>STPSIVIASAARTAVGSFNGAFANTPAHELGATVISAVLERAGVAAGEVNEVILGQVLPAGEGQNPARQAAMKAGVPQEATAWGMNQLCGSGLRAVALGMQQIATGDASIIVAGGMESMSMAPHCAHLRGGVKMGDFKMIDTMIKDGLTDAFYGYHMGTTAENVAKQWQLSRDEQDAFAVASQNKAEAAQKDGRFKDEIVPFIVKGRKGDITVDADEYIRHGATLDSMAKLRPAFDKEGTVTAGNASGLNDGAAAALLMSEAEAS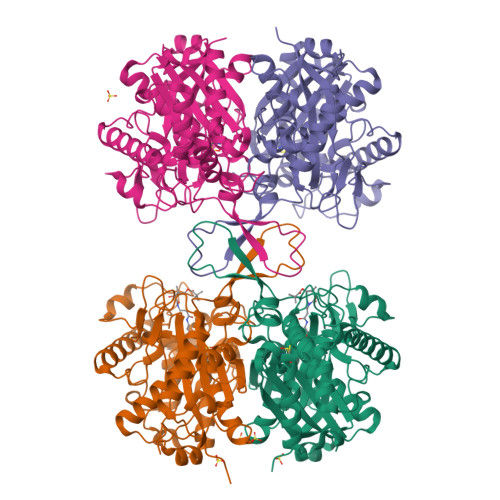RRGIQPLGRIVSWATVGVDPKVMGTGPIPASRKALERAGWKIGDLDLVEANEAFAAQACAVNKDLGWDPSIVNVNGGAIAIGHPIGASGARILNTLLFEMKRRGARKGLATLCIGGGMGVAMCIESL[4x]>[3x]MGSMSSPSTSSSGTVRMNAPVFYFAASFILIFGIIVIAFPQASGAWLLAAQNWAANTVGWYYMMVMTLYLVFVVVTALSGFGKIKLGADHDEPEFSYLSWAGMLFAAGISITLFFFCVSEPLTHLLQPPQGEGGTAEAARQGMQLLFLHWGLHGWGVFAFVGMALAYFAYRHNLPLALRSALYPLIGKRINGPIGYAVDGFGIIATIFGLGADMGFGVLHLNSGLDYLFGVPHTQWIQVGLITLMMGAAILVAIAGVDKGVRVMSDINMLLACALLLFVLFAGPTQHLLNTLVQNIGDYLGALPSKSFDVYAYNKPSDWLGGWTVFYWAWWIAWAPFVGLFIARISRGRTIREFVFGVLLIPLGFTLAWMSIFGNSAIDQVLNHGMAALGQSAIDDPSMTLYLLLETYPWS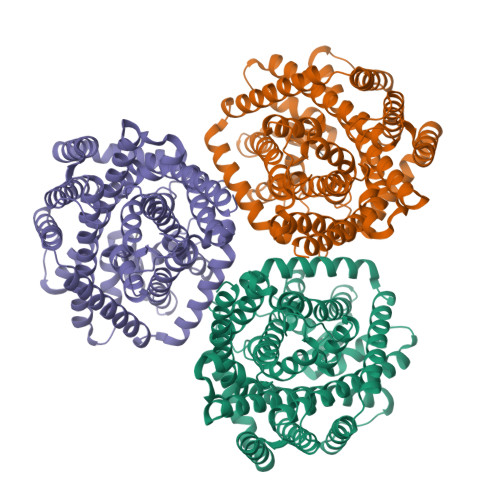KTVIAVTVFISFVFFVTSADSGTVVLSTLSAKGGNPDEDGPKWLRVFWGVATALITSGLLFSGSIDALKSAVVLTSLPFSLILLLMMWGLHKAFVMESQRQIAQLYSLAPVSGSRRGGWRQRLSQAVHYPSRDEVYRFLDQTVRPAIDEVTAVFVEKGLNVVNVPDPSNDSVTLEIGHGEERPFIYQVQMKGFFTPSFARGGMGSKQLNNRRYYRAEVHLSEGSQDYDLVGYTKEQVINDVLDQYERHMQFLHLVRGSGSGSGSGSWSHPQFEK> MKPFNLTVAAKADLRDI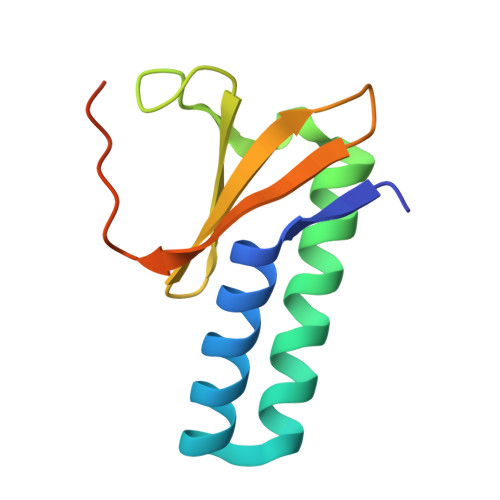ALFTQRRWGKEQRNVYLKQFDDSFWLLAENPDIGKSCDEIREGYRKFPQGSHVIFYQQTGSQQIRVIRILHKSMDVNPIFGAHHHHHH> MYLFMHLCMCFCMISSSQKKEKLNKGKNKQIKLNKKKEKQNKKIEIIKKEKERRSNPQMISKTQAFARLFQLSSKSFSTVKGGNLYTWGQYASGTGFETASAVPRKVDYFSGNVSKVAMGPYHTAVITNDGSLYTFGWGQNGALGNGAKEFQLSPSGNLYTWGQYASGTGFETASAVPRKVDYFSGNVSKVAMGPYHTAVITNDGSLYTFGWGQNGALGNGAKEFQLSPSPVSFFNDKKLKVKDVVVGESYTIAVTENGEVYSWGYGGEPSSKINLDFFRNAILPQRCGALGSGDNKNRLTPQQIANLKADGYKNIS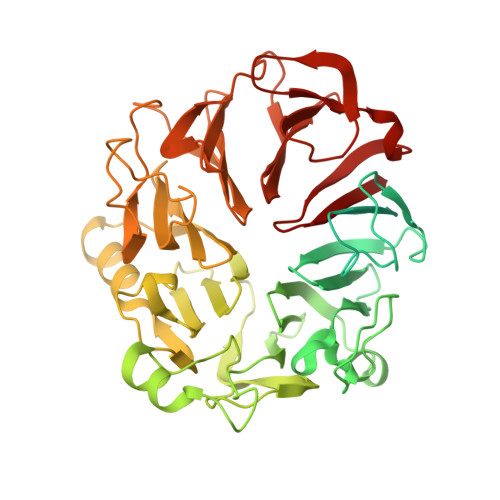GGDNFATLVNQSGEVINWGTGLFGSLGNGSDYPLFTPEVNAYFKHLKEHEGLTVQSIKSAGHFSAALLSNGKLYTFGVNTQGQLGIRENLGHNTDQNARLPTPVVDRHFVGQKVVDFEVGENTLVFLTDKNEVFFSGLELAYQPIRWEIPTDKKIVKLAASKDTFAAVTETGKIYQFNEFVGVSTNEVGNDYNVADSKAFEGKVVDLGGSYGIRFAIVN One key molecule in this process is an enzyme named D-aminoacyl-tRNA deacylase (DTD), which hydrolyses D-amino acids attached to tRNA molecules (a D-aminoacyl-tRNA). Here, we show that besides acting on D-aminoacyl-tRNA, DTD also efficiently hydrolyses the achiral glycine attached to tRNA—glycyl-tRNA(Gly)—as DTD’s active site pocket cannot discriminate between D-amino acids and glycine. Thus, DTD is designed to reject substrates with L-chirality, rather than target substrates with D-chirality. An invariant, cross-subunit Gly-cisPro motif in DTD, inserted into the active site of the dimeric counterpart, is responsible for selectively capturing the chiral centre of D-aminoacyl-tRNA.

We solved the co-crystal structure of PfDTD with Gly3AA at 2.1 Å resolution in P21 space group. The crystal form had eight monomers in the asymmetric unit and, therefore, allowed us to compare eight independent observations of glycine captured by DTD’s proofreading site. It was intriguing to find that the electron density for the glycyl moiety was weaker when compared to that for adenine and ribose, indicating an inherent flexibility of glycine when it sits in the active site pocket. However, it is important to note that the carbonyl oxygen of glycine is rigidly fixed by a DTD fold-specific interaction with main chain N of Phe89 and by its interaction with Nε of Gln88. Thus, the flexibility in glycine was observed only for its α-NH2 group. Analysis of the electron density maps revealed that the α-NH2 group has a preference for the flipped orientation (i.e., the position in which Cβ was seen in D-Tyr3AA complexes), despite its inherent flexibility. Consequently, we placed the α-NH2 group in the flipped orientation in all eight monomers before the final round of refinement. On the other hand, if there were any selection of the amino group of D-amino acids, as observed in the case of D-Tyr3AA complexes, the amino group of glycine moiety in Gly3AA complex would be expected to occupy the same position. In contrast, it prefers majorly the position occupied by the Cβ in D-Tyr3AA complexes, clearly showing a lack of strong selection of the amino group in the opposite orientation. In the second mutant, an alanine (EcDTD Ala102 and PfDTD Ala112) was replaced by a bulkier phenylalanine to sterically abrogate the binding of adenine in the pocket. Both phenylalanine-to-alanine and alanine-to-phenylalanine mutants of EcDTD as well as PfDTD were found to be biochemically inactive on Gly-tRNAGly, thereby validating that the mode of ligand binding as observed in the crystal structure represents the true binding of the actual, full-size substrate (i.e., Gly-tRNAGly).

>MRVVIQRVKGAILSVRKENIGENEKELEIISEIKNGLICFLGIHKNDTWEDALYIIRKCLNLRLWNNDNKTWDKNVKDLNYELLIVSQFTLFGNTKKGNKPDFHLAKEPNEALIFYNKIIDEFKKQYNDDKIKIGKFGNYMNIDVTNDGPVTIYIDTHDINLNK[8x]> MSADAQSFLNRVCGVSAARLTPCGTGTSTDVVYRAFDIYNDKVAGFAKFLKTNCCRFQEKDEDDNLIDSYFVVKRHTFSNYQHEETIYNLLKDCPAVAKHDFFKFRIDGDMVPHISRQRLTKYTMADLVYALRHFDEGNCDTLKEILVTYNCCDDDYFNKKDWYDFVENPDILRVYANLGERVRQALLKTVQFCDAMRNAGIVGVLTLDNQDLNGNWYDFGDFIQTTPGSGVPVVDSYYSLLMPILTLTRALTAESHVDTDLTKPYIKWDLLKYDFTEERLKLFDRYFKYWDQTYHPNCVNCLDDRCILHCANFNVLFSTVFPPTSFGPLVRKIFVDGVPFVVSTGYHFRELGVVHNQDVNLHSSRLSFKELLVYAADPAMHAASGNLLLDKRTTCFSVAALTNNVAFQTVKP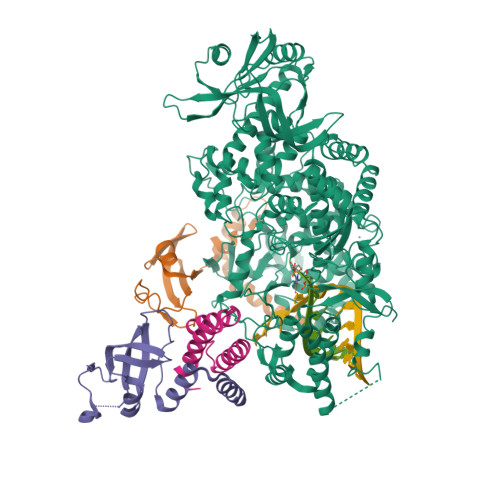GNFNKDFYDFAVSKGFFKEGSSVELKHFFFAQDGNAAISDYDYYRYNLPTMCDIRQLLFVVEVVDKYFDCYDGGCINANQVIVNNLDKSAGFPFNKWGKARLYYDSMSYEDQDALFAYTKRNVIPTITQMNLKYAISAKNRARTVAGVSICSTMTNRQFHQKLLKSIAATRGATVVIGTSKFYGGWHNMLKTVYSDVENPHLMGWDYPKCDRAMPNMLRIMASLVLARKHTTCCSLSHRFYRLANECAQVLSEMVMCGGSLYVKPGGTSSGDATTAYANSVFNICQAVTANVNALLSTDGNKIADKYVRNLQHRLYECLYRNRDVDTDFVNEFYAYLRKHFSMMILSDDAVVCFNSTYASQGLVASIKNFKSVLYYQNNVFMSEAKCWTETDLTKGPHEFCSQHTMLVKQGDDYVYLPYPDPSRILGAGCFVDDIVKTDGTLMIERFVSLAIDAYPLTKHPNQEYADVFHLYLQYIRKLHDELTGHMLDMYSVMLTNDNTSRYWEPEFYEAMYTPHTVLQGGSENLYFQG;>MAIASEFSSLPSYAAFATAQEAYEQAVANGDSEVVLKKLKKSLNVAKSEFDRDAAMQRKLEKMADQAMTQMYKQARSEDKRAKVTSAMQTMLFTMLRKLDNDALNNIINNARDGCVPLNIIPLTTAAKLMVVIPDYNTYKNTCDGTTFTYASALWEIQQVVDADSKIVQLSEISMDNSPNLAWPLIVTALRANSAVKLQ[2x];> MSKMSDVKCTSVVLLSVLQQLRVESSSKLWAQCVQLHNDILLAKDTTEAFEKMVSLLSVLLSMQGAVDINKLCEEMLDNRATLQ>SNAMPFLPDPGEPSPLKVVIAGAGYVGTCLAVTLAGRGAEVVAVDSDPGTVADLRAGRCRLPEPGLAGAVRDLAATGRLTASTSYDPVGAADVVIVTVGTPTDAGHEMVTDQLVAACEQIAPRLRAGQLVILKSTVSPGTTRTLVAPLLESGGLVHERDFGLAFCPERLAEGVALAQVRTLPVVVGGCGPRSAAAAERFWRSALGVDVRQVPSAESAEVVKLATNWWIDANVAIANELARYCAVLGVDVLDVIGAANTLPKGSSMVNLLLPGVGVGGSCLTKDPWMAWRDGRDRGVSLRTVETARAVNDDMPRHTAAVIADELVKLGRDRNDTTIAVLGAAFKNDTGDVRNTPVRGVVAALRDSGFRVRIFDPLADPAEIVARFGTAPAASLDEAVSGAGCLAFLAGHRQFHELDFGALAERVDEPCLVF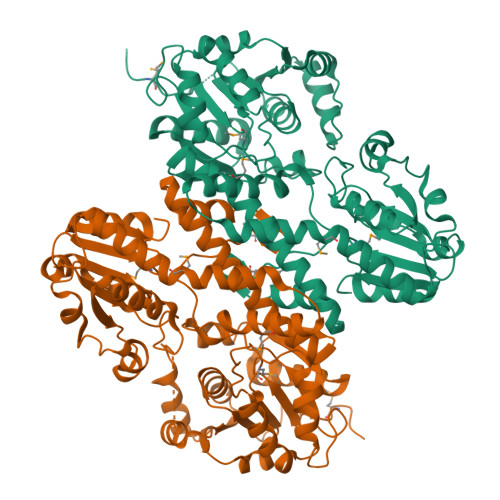DGRMHLPPARIRELHRFGFAYRGIGR[2x]>[10x]ENRPVALITMATGYVGPALARTMADRGFDLVLHGTAGDGTMVGVEESFDSQIADLAKRGADVLTISDVDLTTRTGNQSMIERVLERFGRLDSACLVTGLIVTG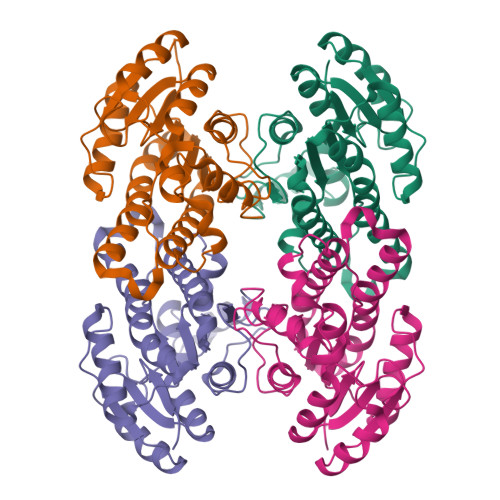KFLDMTDDQWAKVKAWNLDMVFHGLQAVLPPMVAAGAGQCVVFTSATGGRPDPMVSIYGGTRAGANGIVRAVGLEHARHGVQVNAIGTNYMDFPGFLKASRADGDPERRAMIEAQVPLRRLGTMDELSSVTAGLLDGSNRFQTGQFFDFSGGWGA>ADYDLKFGMNAGTSSNEYKAAEMFAKEVKEKSQGKIEISLYPSSQLGDDRAMLKQLKDGSLDFTFAESARFQLFYPEAAVFALPYVISNYNVAQKALFDTEFGKDLIKKMDKDLGVTLLSQAYNGTRQTTSNRAINSIADMKGLKLRVPNAATNLAY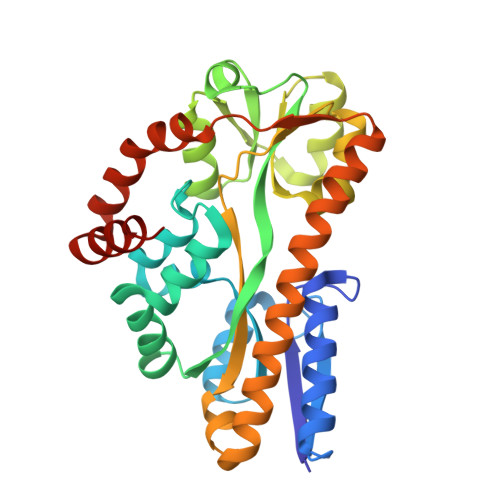AKYVGASPTPMAFSEVYLALQTNAVDGQENPLAAVQAQKFYEVQKFLAMTNHILNDQLYLVSNETYKELPEDLQKVVKDAAENAAKYHTKLFVDGEKDLVTFFEKQGVKITHPDLVPFKESMKPYYAEFVKQTGQKGESALKQIEAINP[4x]>[2x]MHHHHHHSWSPSLTTQTCGAWEMKERLGTGGFGNVIRWHNQETGEQIAIKQCRQELSPRNRERWCLEIQIMRRLTHPNVVAARDVPEGMQNLAPNDLPLLAMEYCQGGDLRKYLNQFENCCGLREGAILTLLSDIASALRYLHENRIIHRDLKPENIVLQQGE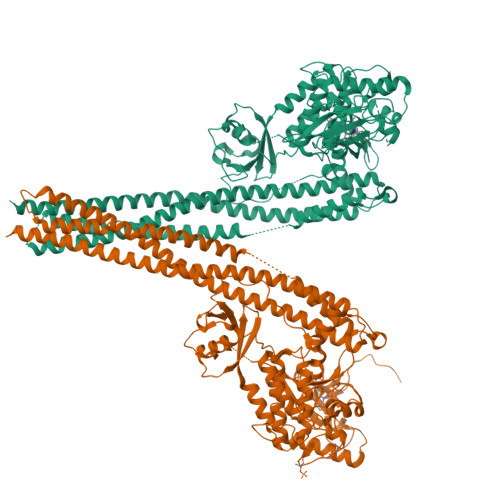QRLIHKIIDLGYAKELDQGSLCTSFVGTLQYLAPELLEQQKYTVTVDYWSFGTLAFECITGFRPFLPNWQPVQWHSKVRQKSEVDIVVSEDLNGTVKFSSSLPYPNNLNSVLAERLEKWLQLMLMWHPRQRGTDPTYGPNGCFKALDDILNLKLVHILNMVTGTIHTYPVTEDESLQSLKARIQQDTGIPEEDQELLQEAGLALIPDKPATQCISDGKLNEGHTLDMDLVFLFDNSKITYETQISPRPQPESVSCILQEPKRNLAFFQLRKVWGQVWHSIQTLKEDCNRLQQGQRAAMMNLLRNNSCLSKMKNSMASMSQQLKAKLDFFKTSIQIDLEKYSEQTEFGITSDKLLLAWREMEQAVELCGRENEVKLLVERMMALQTDIVDLQRSPMGRKQGGTLDDLEEQARELYRRLREKPRDQRTEGDSQEMVRLLLQAIQSFEKKVRVIYTQLSKTVVCKQKALELLPKVEEVVSLMNEDEKTVVRLQEKRQKELWNLLKIACSKSPGRPLN> SMTSSANEDMPVERILEAELAVEPKTETYVEANMGLNPSS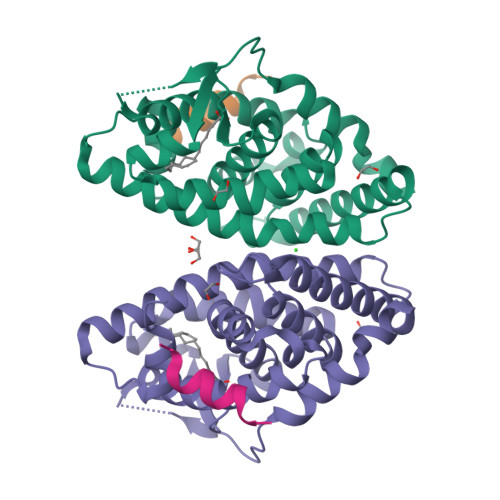PNDPVTNICQAADKQLFTLVEWAKRIPHFSELPLDDQVILLRAGWNELLIASFSHRSIAVKDGILLATGLHVHRNSAHSAGVGAIFDRVLTELVSKMRDMQMDKTELGCLRAIVLFNPDSKGLSNPAEVEALREKVYASLEAYCKHKYPEQPGRFAKLLLRLPALRSIGLKCLEHLFFFKLIGDTPIDTFLMEMLEAPHQMT;> KHKILHRLLQDSSY>[2x]MQAGPALMRIL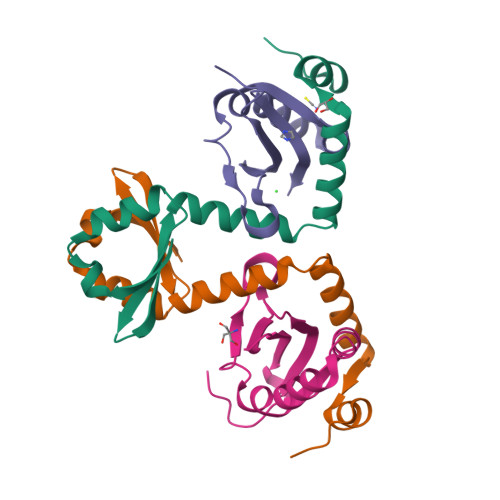PISTIKGKLNEFVDAVSSTQDQITITKNGAPAAVLVGADEWESLQETLYWLAQPGIRESIAEADADIASGRTYGEDEIRAEFGVPRRPHDYKDDDDK;>MAHHHHHHVDDDDKMVPYTVRFTTTARRDLHKLPPRILAAVVEFAFGDLSREPLRVGKPLRRELAGTFSARRGTYRLLYRIDDEHTTVVILRVDHRADIYRR[2x]>[2x]MGGSHHHHHHENLYFQGANLRKVLISDSLDPCCRKILQDGGLQVVEKQNLSKEELIAELQDCEGLIVRSATKVTADVINAAEKLQVVGRAGTGVDNVDLEAATRKGILVMN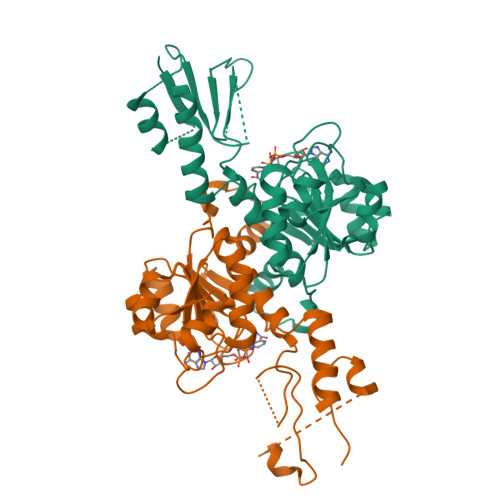TPNGNSLSAAELTCGMIMCLARQIPQATASMKDGKWERKKFMGTELNGKTLGILGLGRIGREVATRMQSFGMKTIGYDPIISPEVSASFGVQQLPLEEIWPLCDFITVHTPLLPSTTGLLNDNTFAQCKKGVRVVNCARGGIVDEGALLRALQSGQCAGAALDVFTEEPPRDRALVDHENVISCPHLGASTKEAQSRCGEEIAVQFVDMVKGKSLTGV> MAHHHHHHVDDDDKMTITSSLDVRPEIKQAVTVRPGMCGPGSLFVGQLGDWTWETVSAQCDTDVFAA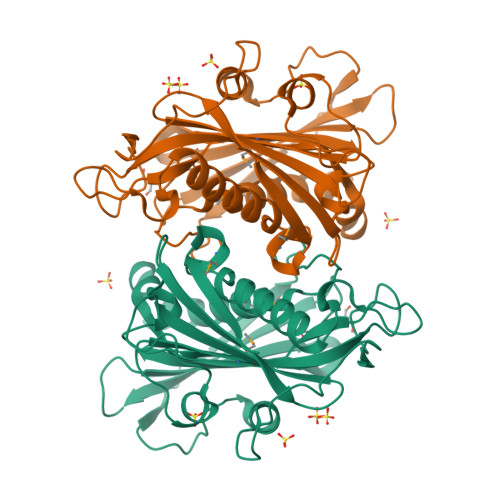RDASGNPTYLAFYYFRVRGGRELHPGSLTFGDRLTVTSGCYDQGTESVLTLHRIDRAGSDDAQRPLDLHEFYERPRDGSLYVENFNRWVTRSAPGSNEDLVKSSPPGFRNDGLPQLPAAYSPRAVYREARTAHTFRALDEPGFRLLPDTVEVEHPVDIVRDVNGVGLLYFASYFSMVDKAALALWRRLGRSDRAFLRRVVVDQQMCYLGNADLDSVLTLGARVRVSTETPGEELVDVVISDRDSGRVIAVSTLHTQHDAHDPKGEA>CGCAAGCTGGCG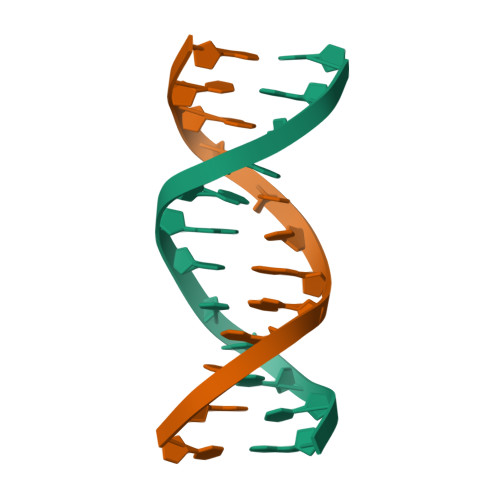[2x]>MHHHHHHMSTTVEKIKAIEDEMARTQKNKATSFHLGQLKAKLAKLRRELLTSASSGSGGGAGIGFDVARTGVASVGFVGFPSVGKSTLLSKLTGTESEAAEYEFTTLVTVPGVIRYKGAKIQMLDLPGIIDGAKDGRGRGKQVIAVARTCNLLFIILDVNKPLHHKQIIEKELEGVGIRLNKTPPDILIKKKEKGGISITNTVPLTHLGNDEIRAVMSEYRINSAEIAFRCDATVDDLIDVLEASSRRYMPAIYVLNKIDSLSIEELELLYRIPNAVPISSGQDWNLDELLQVMWDRLNLVRIYTKPKGQIPDFTDPVVLRSDRCSVKDFCNQIHKSLVDDFRNALVYGSSVKHQPQYVGLSHILEDEDVVTILKK[2x];>[2x]MEQKRLERESLEKQPKITLEEFIETERGKLDKSKLTPITIANFAQWKKDHVIAKINAEKKLSSKRKPTGREIILKMSAENKSFETDNADMPDDVTQGS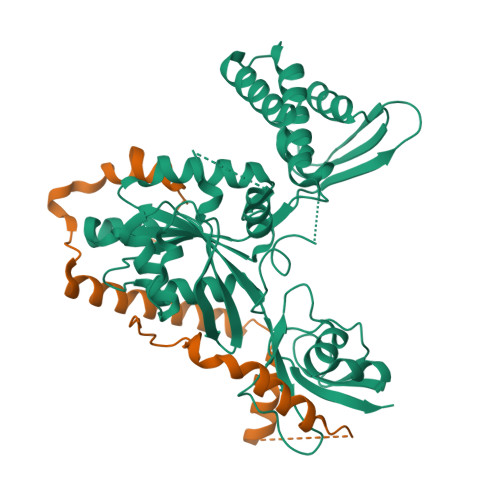AWDLTEFTDALKKADHQDDGGIKDYGDGSNPTFDIKKANSATLA>PPYTVVYFPVRGRSAALRMLLADQGQSWKEEVVTVETWQEGSLKASALYGQLPKFQDGDLTLYQSNTILRHLGRTLGLYGKDQQEAALVDMVNDGVEDLRAKYISLIYTNYEAGKDDYVKALPGQLKPFETLLSQNQGGKTFIVGDQISFADYNLLDLLLIHEVLAPG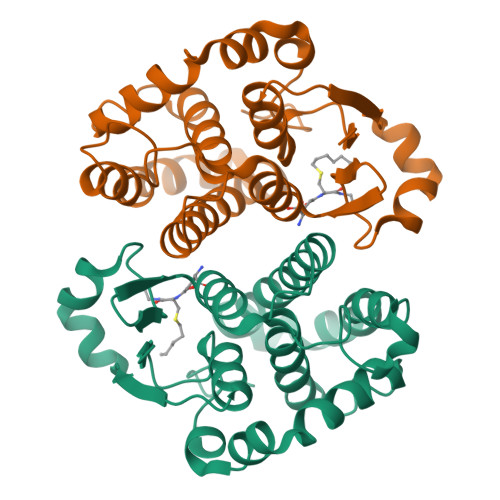SLDAFPLLSAYVGRLSARPKLKAFLASPEYVNLPINGNGKQ[2x]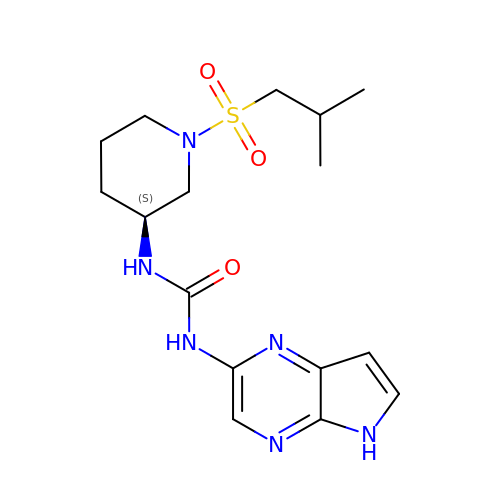1-{(3S)-1-[(2-methylpropyl)sulfonyl]piperidin-3-yl}-3-(5H-pyrrolo[2,3-b]pyrazin-2-yl)urea | C16 H24 N6 O3 S | UTTDMGAEOAWZGU-LBPRGKRZSA-N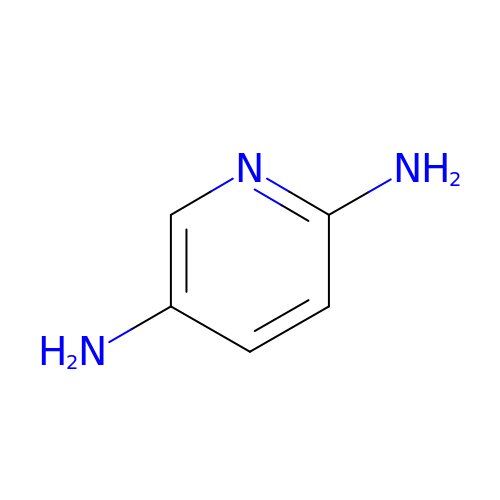PYRIDINE-2,5-DIAMINE | C5 H7 N3 | MIROPXUFDXCYLG-UHFFFAOYSA-N6-[(5S,9R)-9-(4-cyanophenyl)-3-(3,5-dichlorophenyl)-1-methyl-2,4-dioxo-1,3,7-triazaspiro[4.4]non-7-yl]pyridine-3-carboxylic 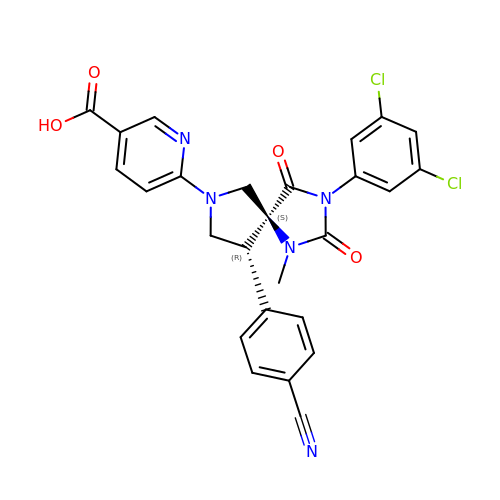acid | C26 H19 Cl2 N5 O4 | LILGMDXLRPEBNH-HFZDXXHNSA-N5-azanyl-3-[1-(pyridin-2-ylmethyl)indol-6-yl]-1~{H}-pyrazole-4-carbonitrile 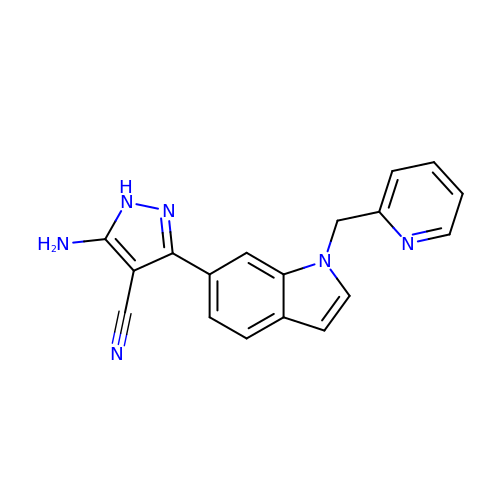| C18 H14 N6 | OGAVRMBWGWENPE-UHFFFAOYSA-N>[7x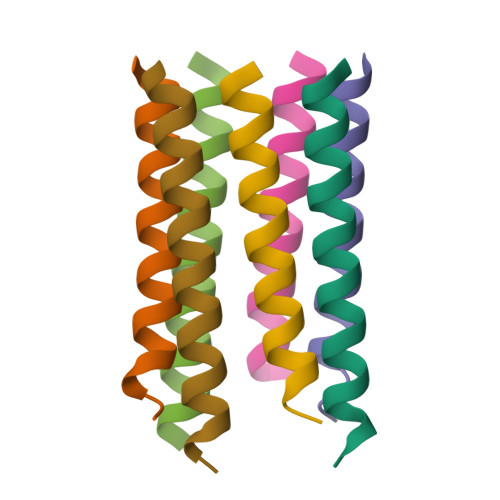]XGEIAKALREIAKALREXAWAHREEAKALRG2-(3-NITROPHENYL)ACETIC ACID | C8 H7 N O4 | 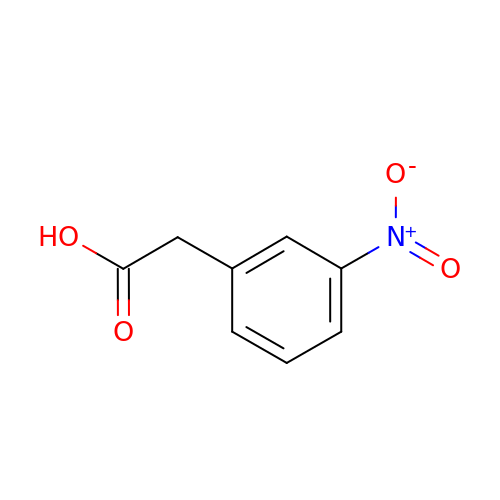WUKHOVCMWXMOOA-UHFFFAOYSA-N> RPEIWIAQELRRIGDE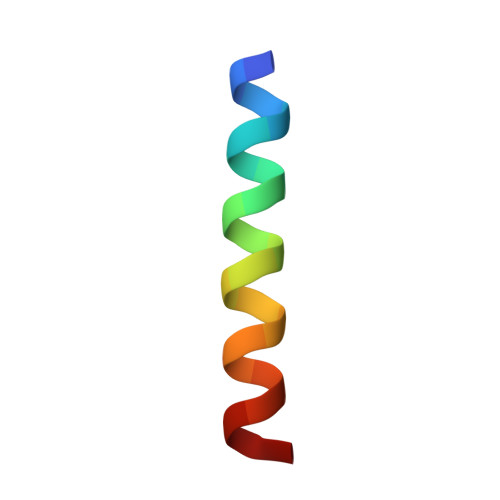ENAYYR However, because of the intrinsic flexibility and irregularity of loop regions, organizing multiple structured loops at protein functional sites has been very difficult to achieve by de novo protein design. Here we describe a solution to this problem that designs tandem repeat proteins with structured loops (9–14 residues) buttressed by extensive hydrogen bonding interactions. Experimental characterization shows that the designs are monodisperse, highly soluble, folded and thermally stable. Crystal structures are in close agreement with the design models, with the loops structured and buttressed as designed.

The in silico validated designs span a diverse range of shapes with different repeat protein curvatures and loop geometries and adopt multiple loop buttressing strategies using loop–helix hydrogen bond networks and loop–loop bidentate hydrogen bonds. From a fundamental design perspective, the crystal structures presented here show that computational protein design has advanced to the point that proteins with multiple ordered long loops can now be designed. Key to this success was the design of dense networks of hydrogen bonding and nonpolar interactions within and between the loops and between the loops and the underlying secondary structural elements.

>[2x]METPLLELIAIVRQGSEEQQKSALEQLKRLLEAGADPNAADNAGKTPLLLLIEIVRQGSEEQQKAALELLKLLLEAGADPNAADNAGKTPLLLLIEIVRQGSEEQQKAALELLKLLLEAGADPNAADNAGKTPLLLLIEIVRQGSEEQQKAALELLKLLLEAGADPNAADNAGQTPQQLLKAIERQGSEEQQKAAKELLKLLEEAGGSWGHHHHHH> MDSTKEKCDSYKDDLLLRMGLNDNKAGMEGLDKEKINKIIMEATKGSRFYGNELKKEKQVNQRIENMMQQKAQITSQQLRKAQLQVDRFAMELEQSRNLSNTIVHIDMDAFYAAVEMRDNPELKDKPIAVGSMSMLSTSNYHARRFGVRAAMPGFIAKRLCPQLIIVPPNFDKYRAVSKEVKEILADYDPNFMAMSLDEAYLNITKHLEERQNWPEDKRRYFIKMGSSVENDNPGKEVNKLSEHERSISPLLFEESPSDVQPPGDPFQVNFEEQNNPQILQNSVVFGTSAQEVVKEIRFRIEQKTTLTASAGIAPNTMLAKVCSDKNKPNGQYQILPNRQAVMDFIKDLPIRKVSGIGKVTEKMLKALGIITCTELYQQRALLSLLFSETSWHYFLHISLGLGSTHLTRDGERKSMSVERTFSEINKAEEQYSLCQELCSELAQDLQKERLKGRTVTIKLKNVNFEVKTRASTVSSVVSTAEEIFAIAKELLKTEIDADFPHPLRLRLMGVRISSFPNEEDRKHQQRSIIGFLQAGNQALSATECTLEKTDKDKFVKPLEMSHKKSFFDKKRSERKWSHQDTFKCEAVNKQSFQTSQPFQVLKKKMNENLEISENSDDCQIL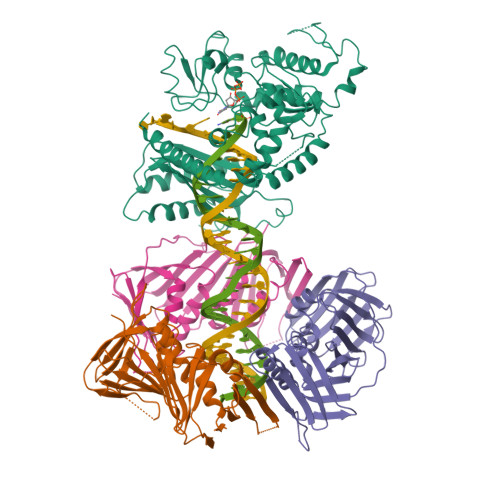TCPVCFRAQGCISLEALNKHVDECLDGPSISENFKMFSCSHVSATKVNKKENVPASSLCEKQDYEAHPKIKEISSVDCIALVDTIDNSSKAESIDALSNKHSKEECSSLPSKSFNIEHCHQNSSSTVSLENEDVGSFRQEYRQPYLCEVKTGQALVCPVCNVEQKTSDLTLFNVHVDVCLNKSFIQELRKDKFNPVNQPKESSRSTGSSSGVQKAVTRTKRPGLMTKYSTSKKIKPNNPKHTLDIFFK;>GPHMFEARLVQGSILKKVLEALKDLINEACWDISSSGVNLQSMDSSHVSLVQLTLRSEGFDTYRCDRNLAMGVNLTSMSKILKCAGNEDIITLRAEDNADTLALVFEAPNQEKVSDYEMKLMDLDVEQLGIPEQEYSCVVKMPSGEFARICRDLSHIGDAVVISCAKDGVKFSASGELGNGNIKLSQTSNVDKEEEAVTIEMNEPVQLTFALRYLNFFTKATPLSSTVTLSMSADVPLVVEYKIADMGHLKYYLAPKIEDEEGS[3x]>[2x]HPIKETVVEEPVDITPYLDQLDESLRDKVLQLQKGSDTEAQCEVMQEIVDQVLEEDFDSEQLSVLASCLQELFKAHFRGEVLPEEITEESLEESVGKPLYLIFRNLCQMQEDNSSFSLLLDLLSELYQKQPKIGYHLLYYLRASKAAAGKMNLYESFAQATQLGDLHTCLMMDMKACQEDDVRLLCHLTPSIYTEFPDETLRSGELLNM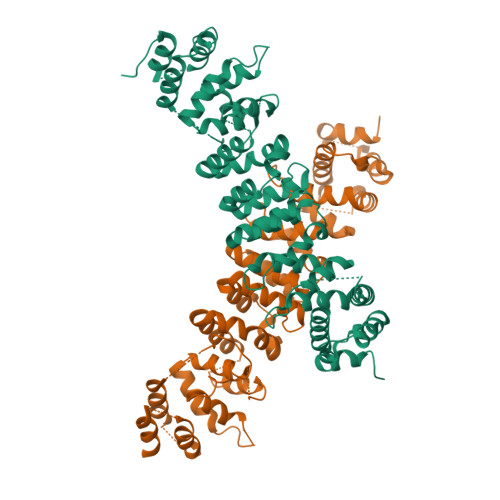IVAVIDSAQLQELVCHVMMGNLVMFRKDSVLNILIQSLDWETFEQYCAWQLFLAHNIPLETIIPILQHLKYKEHPEALSCLLLQLRREKPSEEMVKMVLSRPCHPDDQFTTSILRHWCMKHDELLAEHIKSLLIKNNSLPRKRQSLRSSSSKLAQLTLEQILEHLDNLRLNLTNTKQNFFSQTPILQALQHVQASCDEAHKMKFSDLFSLAEEY>[4x]GADLADRFAELERRYDARLGVYVPATGTTAAIEYRADERFAFCSTFKAPLVAAVLHQNPLTHLDKLITYTSDDIRSISPVAQQHVQTGMTIGQLCDAAIRYSDGTAANLLLADLGGPGGGTAAFTGYLRSLGDTVSRLDAEEPELNRDPPGDERDTTTPHAIALVLQQLVLGNALPPDKRALLTDWMARNTTGAKRIRAGFPADWKVIDKTGTGDYGRANDIAVVWSPTGVPYVVAVMSDRAGGGYDAEPREALLAEAATCVAGVLA

Beta(β)-lactamases are bacterial enzymes that provide multi-drug resistance to β-lactam antibiotics. Mtb β-lactamase (BlaC) is a broad-spectrum Ambler class A3 β-lactamase capable of hydrolyzing all classes of β-lactam antibiotics used for the treatment of tuberculosis. Sulbactam (SUB), clavulanate and tazobactam, all β-lactam based suicide inhibitors, irreversibly bind to β-lactamases and block their activity. Here, we report in atomic detail (between 2.2 and 2.7 Å resolution) by room-temperature, time-resolved crystallography with millisecond time-resolution (with timepoints between 3 ms and 700 ms) how the Mycobacterium tuberculosis enzyme BlaC is inhibited by sulbactam (SUB).

Due to its smaller size, SUB should diffuse faster into the crystals than CEF, and the signature of an enzyme inhibitor complex is expected to appear at the earliest time points (3 ms and 6 ms). Nevertheless, contrary to expectations based on the size of the SUB, no electron density is present at the earliest time points. This can be explained by the smaller second-order binding coefficient, kncov (1.5 mM−1 s−1 for SUB compared to 3.2 mM−1 s−1 for CEF), which prevents the accumulation of electron density at earlier times. At 3, 6, and 15 ms, the DED features near the active site of subunit A are weak. At 6 and 15 ms, density features appear closer toward Ser70. These results could indicate an initial trace of SUB molecules migrating to the active site after being held up by the guardian residues. The guardian residues open the active site after approximately 6 ms, which corresponds to the outside ligand concentration of approximately 35 mM.> MSEKKEARVVINDLLAEQYANAFKAKEEGRPVGWSTSVFPQELAEVFDLNVLYPENQAAGVAAKKGSLELCEIAESKGYSIDLCAYARTNFGLLENGGCEALDMPAPDFLLCCNNICNQVIKWYENISRELDIPLIMIDTTFNNEDEVTQSRIDYIKAQFEEAIKQLEIISGKKFDPKKFEEVMKISAENGRLWKYSMSLPADSSPSPMNGFDLFTYMAVIVCARGKKETTEAFKLLIEELEDNMKTGKSSFRGEEKYRIMMEGIPCWPYIGYKMKTLAKFGVNMTGSVYPHAWALQYEVNDLDGMAVAYSTMFNNVNLDRMTKYRVDSLVEGKCDGAFYHMNRSCKLMSLIQYEMQRRAAEETGLPYAGFDGDQADPRAFTNAQFETRIQGLVEVMEERKKLNRGEI;> MEAILSKMKEVVENPNAAVKKYKSETGKKAIGCFPVYCPEEIIHAAGMLPVGIWGGQTELDLAKQYFPAFACSIMQSCLEYGLKGAYDELSGVIIPGMCDTLICLGQNWKSAVPHIKYISLVHPQNRKLEAGVKYL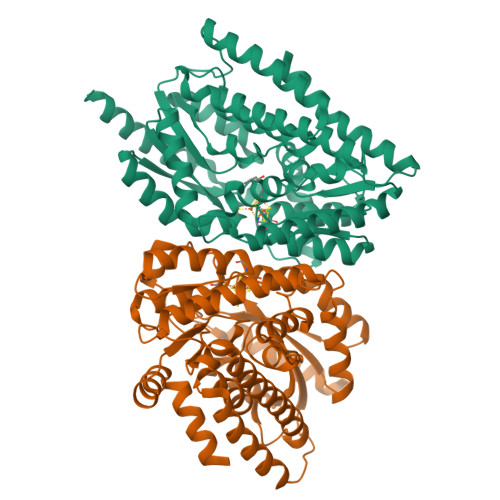ISEYKGVKRELEEICGYEIEEAKIHESIEVYNEHRKTMRDFVEVAYKHSNTIKPSIRSLVIKSGFFMRKEEHTELVKDLIAKLNAMPEEVCSGKKVLLTGILADSKDILDILEDNNISVVADDLAQETRQFRTDVPAGDDALERLARQWSNIEGCSLAYDPKKKRGSLIVDEVKKKDIDGVIFCMMKFCDPEEYDYPLVRKDIEDSGIPTLYVEIDQQTQNNEQARTRIQTFAEMMSLASAWSHPQFEK> MGHHHHHHHHHHSSGHIEGRHMGKNVLLLGSGFVAQPVIDTLAANDDINVTVACRTLANAQALAKPSGSKAISLDVTDDSALDKVLADNDVVISLIPYTFHPNVVKSAIRTKTDVVTSSYISPALRELEPEIVKAGITVMNEIGLDPGIDHLY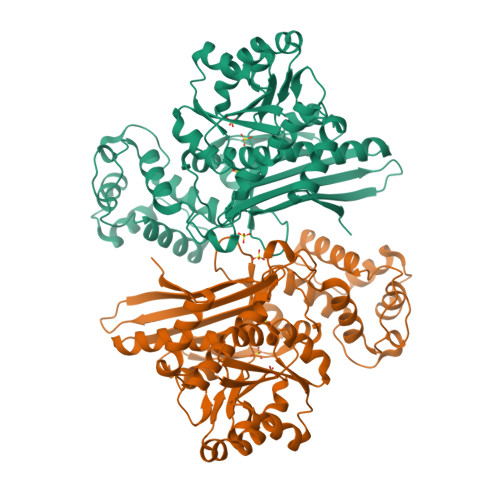AVKTIDEVHRAGGKLKSFLSYCGGLPAPEDSDNPLGYKFSWSSRGVLLALRNSAKYWKDGKIETVSSEDLMATAKPYFIYPGYAFVCYPNRDSTLFKDLYHIPEAETVIRGTLRYQGFPEFVKALVDMGMLKDDANEIFSKPIAWNEALKQYLGAKSTSKEDLIASIDSKATWKDDEDRERILSGFAWLGLFSDAKITPRGNALDTLCARLEELMQYEDNERDMVVLQHKFGIEWADGTTETRTSTLVDYGKVGGYSSMAATVGYPVAIATKFVLDGTIKGPGLLAPYSPEINDPIMKELKDKYGIYLKEKTVA> MMDFLSKTPEPPYYAVIFSSVKSENDTGYGETAERMVSLAADQPGFLGVESVREADGRGITVSYWDSMDAINHWRHHTEHQAAKEKGRSVWYESYAVRVAKVDRQRLFQENTNDLEHHH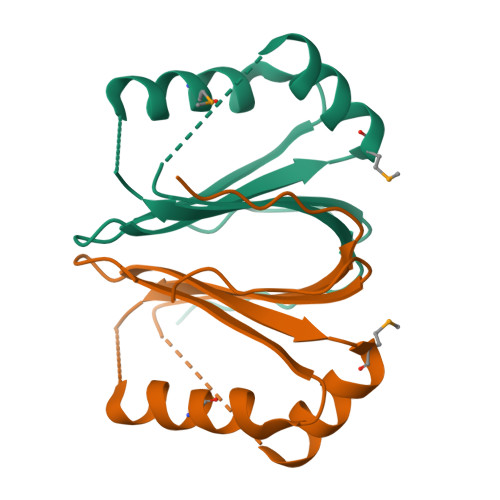HHH>UUGCGUCACCUCGAGCAAGUCGC[2x];> UGCGUCACCUCGAGCAAGUCGC;> GCGUCACCUCGAGC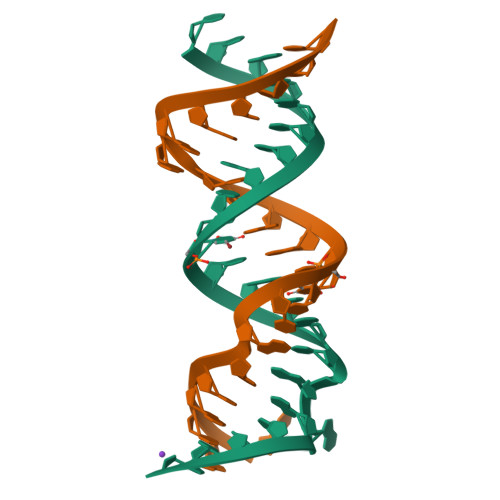AAGUCGC> VKKTIYVNPDSGQNRKVSDRGLTSRDRRRIARWEKRIAYALKNGVTPG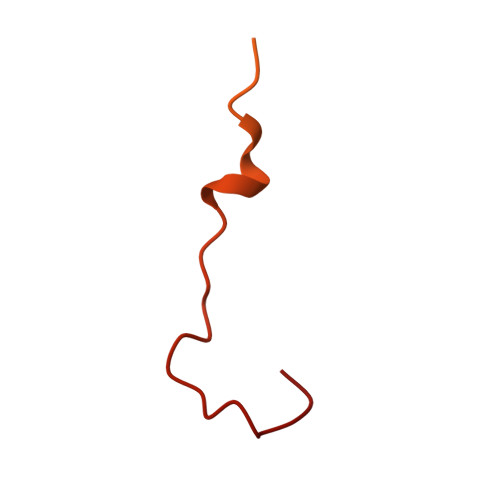FNAIDDGPEYKINEDPMDKVDKALATPFPRDVEKIEDEKYEDVMHRVVNHAHQRNPNKKWS> SVCAEAYNPDEEEDDAESRIIHPKTDDQRNRLQEACKDILLFKNLDPEQMSQVLDAMFEKLVKEGEHVIDQGDDGDNFYVIDRGTFDIYVKCDGVGRCVGNYDNRGSFGELALMYNTPRAATITATSPGALWGLDRVTFRRIIVKNNAKKRKMYESFIESLPFLKSLEVSERLKVVDVIGTK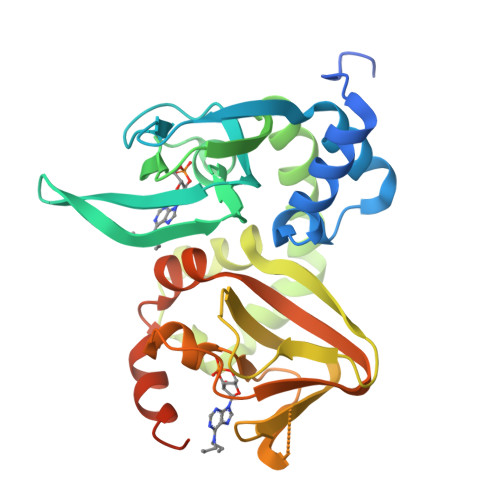VYNDGEQIIAQGDSADSFFIVESGEVRITMKRKGKSDIEENGAVEIARCLRGQYFGELALVTNKPRAASAHAIGTVKCLAMDVQAFERLLGPCMEIMKRNIATYEEQLVALFGTNMDIVEPTA> MDISAPTNTLVNCIATAPMKLSPAITNDANDFNASSQQVYNRLVEFKAGKIEVEPGLAERWEISEDGLVYTFYLRQNVKFHSNKTFSPTRPLNADDVVFSFQRQADKNHPYHNVSAGTYFYF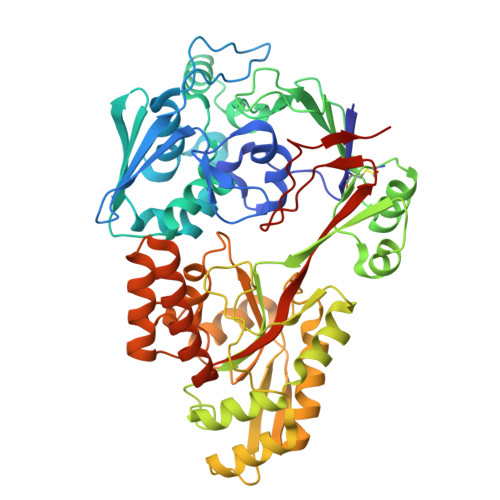NWMNLPSILKSVEKVDDYTVKITLNKPNTPFITTVAMDFLSIYSKEYADQLLAQGKPETLDQQPIGTGPFIFQTNQTDHAVRYTANVDYWKGKADIERLIFSITPDAGTRYAKLKAGECDVIDFPNISDIAQMKKDPQINLLEREGLNLAYIGLNTTKPELNNVKVRQALHHATDKKAIVDAVYQGGGTVATNPFPDAVLGYNPHLPQYEFNLEKAKALLAEAGYPNGFETEIWVQPVVRPSNPNPRRTAEIIQADWAKIGVKAKLVTHEWADFNKRTREGEFAAGTYGWTSRNGDPDNFLFPLFSQANIPGTNYSRWTDEKFEALLASAAQIQDTQTRAKLYQQAVEIFQQNSPIIPFAHSINYVPLNKRVQGFVQNPFGYTAFYGVSLKLEHHHHHH(2S,3AR,4R,6R,6AR)-4-(6-AMINO-9H-PURIN-9-YL)-6-({[(R)-HYDROXY(SULFOOXY)PHOSPHORYL]OXY}METHYL)TETRAHYDROFURO[3,4-D][1,3,2]DIOXAPHOSPHOL-2-OL 2-OXIDE | C10 H13 N5 O12 P2 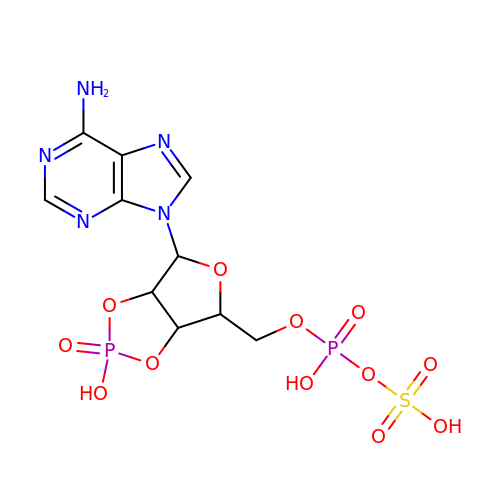S | BOTWXJFMSRDLBQ-KQYNXXCUSA-N>MVRSFIYEPFQIPSGSMMPTLLIGDFILVEKFAYGIKDPIYQKTLIETGHPKRGDIVVFKYPEDPKLDYIKRAVGLPGDKVTYDPVSKELTIQPGCSSGQACENALPVTYSNVEPSDFVQTFSRRNGGEATSGFFEVPKNETKENGIRLSERKETLGDVTHRILTVPIAQDQVGMYYQQPGQQLATWIVPPGQYFMMGDNRDNSADSRYWGFVPEANLVGRATAIWMSFDKQE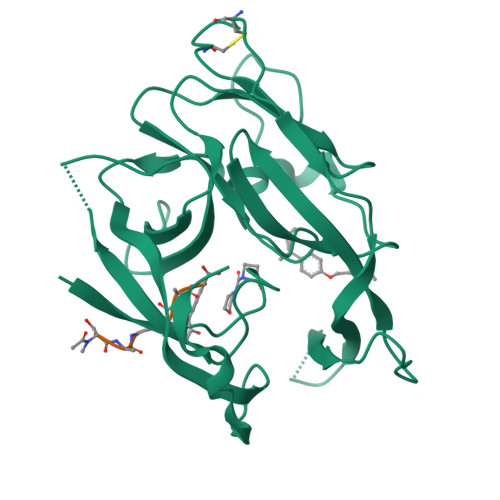GEWPTGLRLSRIGGIH[2x];>[2x]SAGGAY>MPKHEFSVDMTCGGCAEAVSRV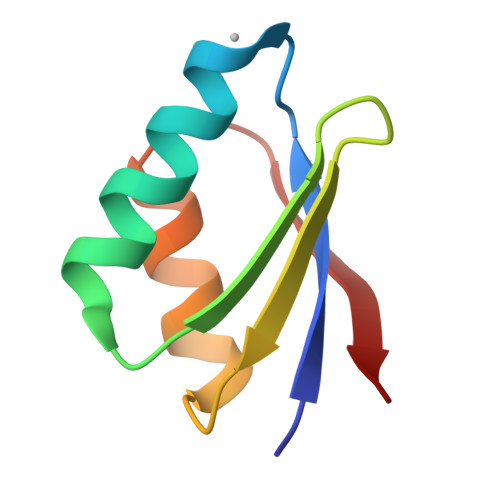LNKLGGVKYDIDLPNKKVCIESEHSMDTLLATLKKTGKTVSYLGLE[4x]>[4x]MYTLNWQPPYDWSWMLGFLAARAVSSVETVADSYYARSLAVGEYRGVVTAIPDIARHTLHINLSAGLEPVAAECLAKMSRLFDLQCNPQIVNGALGRLGAARPGLRLPGCVDAFEQGVRAILGQL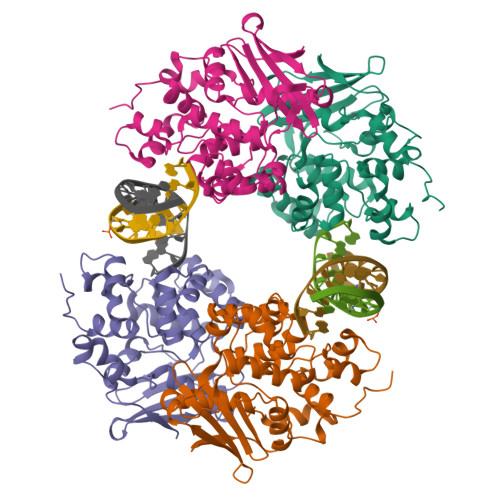VSVAMAAKLTARVAQLYGERLDDFPEYICFPTPQRLAAADPQALKALGMPLKRAEALIHLANAALEGTLPMTIPGDVEQAMKTLQTFPGIGRWTANYFALRGWQAKDVFLPDDYLIKQRFPGMTPAQIRRYAERWKPWRSYALLHIWYTEGWQPDEA The Tol-Pal system is essential for maintaining outer membrane (OM) stability during cell division in Gram-negative bacteria. The inner membrane complex TolQRA harnesses proton motive force (PMF) to establish transient interactions within the periplasm, thereby coordinating cell envelope remodeling and facilitating OM invagination at division sites. TolQ forms a pentameric structure similar to that of MotA and ExbB, exhibiting a volcano-like configuration with a narrow periplasmic end and a wider cytoplasmic base. The pentameric TolQ encapsulates the dimeric TolR through its N-terminal transmembrane helices at the periplasmic end.

To explore the dynamic motion of the TolQRA complex, we aimed to capture its distinct states using styrene-maleic acid (SMA) polymers. Two distinct structural classes with high resolutions were determined at 2.92 and 3.28 Å, respectively, with one class lacking density for TolA (hereafter TolQ5R2) and the other displaying density corresponding to one copy of TolA (hereafter TolQ5R2A). The TolA molecule bound in TolQ5R2A is positioned consistently with its location on the TolQ1 subunit in the nanodisc TolQ5R2A3 structure. The superimposition of the TolQ5R2 and TolQ5R2A structures onto the TolQ5R2A3 structure shows root-mean-square deviation (RMSD) values of 1.31 and 2.52 Å, respectively, based on the alignment of 217 Cα atoms. When viewed from the cytoplasmic side of the pentamer, TolQ5R2A3 features an oval-shaped cytoplasmic opening, TolQ5R2 presents a round opening, and TolQ5R2A displays a split between TolQ1 and TolQ5 as well as between TolQ3 and TolQ4.

>MTDMNILDLFLKASLLVKLIMLILIGFSIASWAIIIQRTRILNAAAREAEAFEDKFWSGIELSRLYQESQGKRDNLTGSEQIFYSGFKEFVRLHRANSHAPEAVVEGASRAMRISMNRELENLETHIPFLGTVGSISPYIGLFGTVWGIMHAFIALGAVKQATLQMVAPGIAEALIATAIGLFAAIPAVMAYNRLNQRVNKLELNYDNFMEEFTAILHRQAFTVSESNKG[5x];>[2x]MARARGRGRRDLKSEINIVPLLDVLLVLLLIFMATAPIITQSVEVDLPDATESQAVSSNDNPPVIVEVSGIGQYTVVVEKDRLERLPPEQVVAEVSSRFKANPKTVFLIGGAKDVPYDEIIKALNLLHSAGVKSVGLMTQPI;> MSKATEQNDKLKRAIIISAVLHVILFAALIWSSFDENIEASAGGGGGSSIDAVMVDSGAVVEQYKRMQSQESSAKRSDEQRKMKEQQAAEELREKQAAEQERLKQLEKERLAAQEQKKQAEEAAKQAELKQKQAEEAAAKAAADAKAKAEADAKAAEEAAKKAAADAKKKAEAEAAKAAAEAQKKAEAAAAALKKKAEAAEAAAAEARKKAATEAAEKAKAEAEKKAAAEKAAADKKAAAEKAAADKKAAEKAAAEKAAADKKAAAEKAAADKKAAAAKAAAEKAAAAKAAAEADDIFGELSSGKNAPKTGGGAKGNNASPAGSGNTKNNGASGADINNYAGQIKSAIESKFYDASSYAGKTCTLRIKLAPDGMLLDIKPEGGDPALCQAALAAAKLAKIPKPPSQAVYEVFKNAPLDFKP>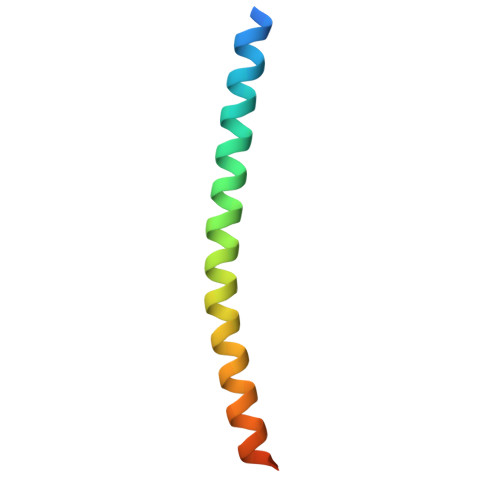 FNSSINNIHEMEIQLKDALEKNQQWLVYDQQREVYVKGLLAKIFELEKKTETAAHSLP(2S,3S)-2-azanyl-4-(2-hydroxy-2-oxoethylamino)-3-oxidanyl-butanoic acid | C6 H12 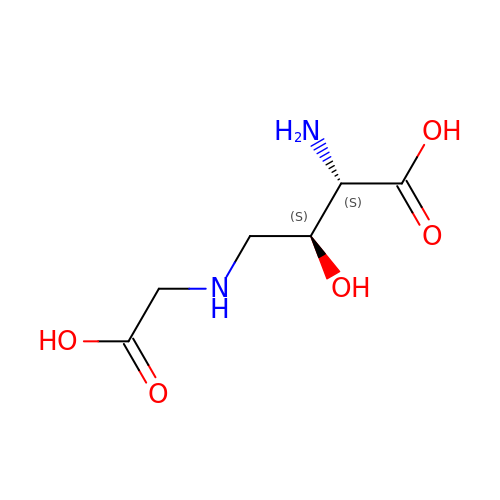N2 O5 | ITNGKQLAUYSKRS-UCORVYFPSA-N6-[2-(3-fluoro-5-{2-[(2R,4S)-4-fluoro-1-methylpyrrolidin-2-yl]ethyl}phenyl)ethyl]-4-methylpyridin-2-amine | C21 H27 F2 N3 | 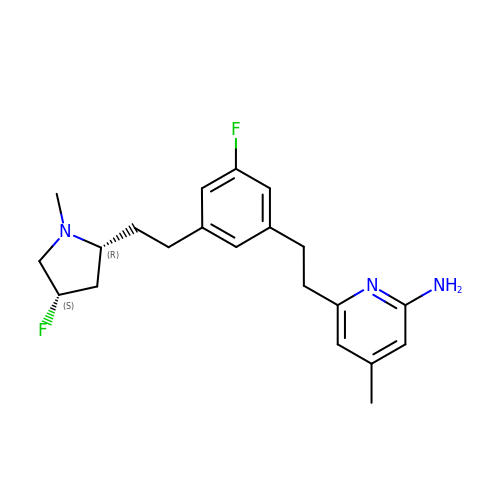ASCMQTSVWSFRKT-AZUAARDMSA-N> MFRGFRPVLAADAVKFQTLYNVLTGKQHLKDQVPVKDCNLTAIFGASWKADLNKWFDSEYAPKLPAAERDSAKKSLDLYLKRVDLTRYTREELTTYGILACGPGKVDALTE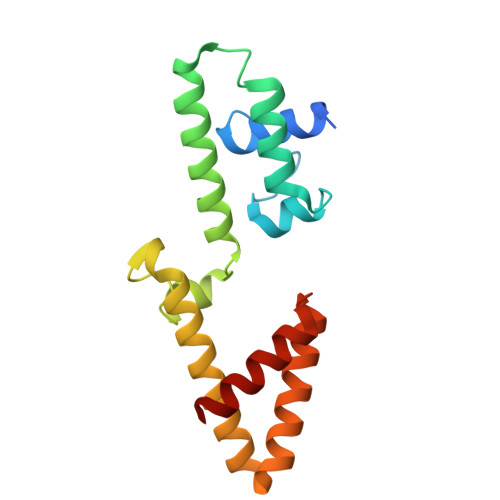KHLLETGKARLEELTAGLGNKDEGVNAFRKEVEQEGKYANWPAEKSKALADKVIAASP> MTVKAPSVTSLRISKLSANQVQVRWDDVGANFYYFVEIAETKTNSGENLPSNQYRWINLGYTANNSFFFDDADPLTTYIIRVATAAQDFEQSDWIYTEEFETFATNAYTFQNMIEMQLANKFIQEKFTLNNSDYVNFNNDTIMAALMNESFQFSPSYVDVSSISNFIIGENEYHEIQGSIQQVCKDINRVYLMESEGILYLFERYQPVVKVSNDKGQTWKAVKLFNDRVGYPLSKTVYYQSANTTYVLGYDKIFY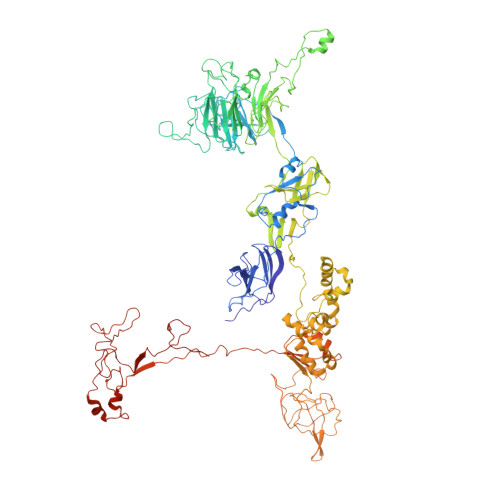GRKSTDVRWSADDVRFSSQDITFAKLGDQLHLGFDVEIFATYATLPANVYRIAEAITCTDDYIYVVARDKVRYIKTSNALIDFDPLSPTYSERLFEPDTMTITGNPKAVCYKMDSICDKVFALIIGEVETLNANPRTSKIIDSADKGIYVLNHDEKTWKRVFGNTEEERRRIQPGYANMSTDGKLVSLSSSNFKFLSDNVVNDPETAAKYQLIGAVKYEFPREWLADKHYHMMAFIADETSDWETFTPQPMKYYAEPFFNWSKKSNTRCWINNSDRAVVVYADLKYTKVIENIPETSPDRLVHEYWDDGDCTIVMPNVKFTGFKKYASGMLFYKASGEIISYYDFNYRVRDTVEIIWKPTEVFLKAFLQNQEHETPWSPEEERGLADPDLRPLIGTMMPDSYLLQDSNFEAFCEAYIQYLSDGYGTQYNNLRNLIRNQYPREEHAWEYLWSEIYKRNIYLNADKRDAVARFFESRSYDFYSTKGIEASYKFLFKVLYNEEVEIEIESGAGTEYDIIVQSDSLTEDLVGQTIYTATGRCNVTYIERSYSNGKLQWTVTIHNLLGRLIAGQEVKAERLPSFEGEIIRGVKGKDLLQNNIDYINRSRSYYVMKIKSNLPSSRWKSDVIRFVHPVGFGFIAITLLTMFINVGLTLKHTETIINKYKNYKWDSGLPTEYADRIAKLTPTGEIEHDSVTGEAIYEPGPMAGVKYPLPDDYNAENNNSIFQGQLPSERRKLMSPLFDASGTTFAQFRDLVNKRLKDNIGNPRDPENPTQVKIDE>MGSSHHHHHHSAALEVLFQGPDYKFWYTQPVPKINDEFNESVNEPFISDNKVEDVRKDEYKLPPGYSWYVCDVKDEKDRSEIYTLLTDNYVEDDDNIFRFNYSAEFLLWALTSPNYLKTWHIGVKYDASNKLIGFISAIPTDICIHKRTIKMAEVNFLCVHKTLRSKRLAPVLIKEITRRINLENIWQAIYTAGVYLPKPVSDARYYHRSINVKKLIEIGFSSLNSRLTMSRAIKLYRVEDTLNIKNMRLMKKKDVEGVHKLLGSYLEQFNLYAVFTKEEIAHWFLPIENVIYTYVNEENGKIKDMISFYSLPSQILGNDKYSTLNAAYSFYNVTTTATFKQLMQDAILLAKRNNFDVFNALEVMQNKSVFEDLKFGEGDESLKYYLYNWKCASFAPAHVGIVLL[3x]

The attachment of myristate to the N-terminal glycine of certain proteins is largely a co-translational modification catalyzed by N-myristoyltransferase (NMT), and involved in protein membrane-localization. Using coenzyme A (CoA)-activated lipid, NMT transfers myristate to the substrate protein, after removal of the initiator methionine, in a predominantly co-translational process (Ritzefeld et al., 2017, Schlott et al., 2018). Pathogen NMT is a validated therapeutic target in numerous infectious diseases including malaria. PvNMT possesses 80% sequence identity and 93% similarity to PfNMT and is an excellent platform for structural studies, while to date PfNMT has proven intractable for X-ray crystallography.

The current study describes identification and validation of the consequence of a single amino acid substitution (G386E) in the substrate-binding pocket of Plasmodium NMT, identified by drug selection of a non-synonymous point mutation in the nmt open reading frame. In contrast to G386, E386 places a large, charged side chain in direct proximity to the nearby Y211 residue. Interestingly, the nearby His213 displays a larger degree of flexibility in the PvNMT[WT] structure, modeled as two possible rotamers (H213a, H213b), whereas the residue adopts a single conformation in the G386E variant (H213a). A preferred conformation (rotamer Y211a) was adopted in both the unliganded PvNMT[WT] and [G386E] enzymes, and, on binding of DDD85646 to PvNMT[WT], Y211 moved only slightly to rotamer Y211b when DDD85646 was bound to PvNMT[G386E]. We found, depending on the inhibitor bound (IMP-1002, DDD85646 or in the apo form), that E386 can adopt up to four distinct occupancies showing its flexible nature. Even though G386E reduces the space in the peptide-binding pocket, the flexibility of Y211, E386, and H213 provides a plausible explanation for why substrate myristoylation is unaffected, leading to no reduction in fitness or change in global myristoylation. There was very little difference in labeling pattern, and therefore no detectable effect of the G386E substitution on global myristoylation, while continuous culture of the two PfNMT[G386E] clones revealed no significant growth defect over six generations as assessed by relative parasitemia, normalized to the WT population. These data provide evidence that enzyme function is not compromised in the G386E variant.>[2x]MTDTDTVEQFIHTIFARVTDDHGRPVDITAALPLLKQILTGYTQEVAEHKFNYIGESAVQFAMHLILADHFSKYENGCLSAIAKKYTVPLQLYKLIGKQIHLKEYVRPVYLKETLDMIVGILFRCYGITAVYKFIQEEFILLVNQDINNANSPKKPSSPSLSTNQADNPVKLLHELIQAKSGTLEAEAHETEDKKWEVKIVAKLNEKALPFSHARTNASKQKAKTEASRDILTYFTNYPDVCQHLQ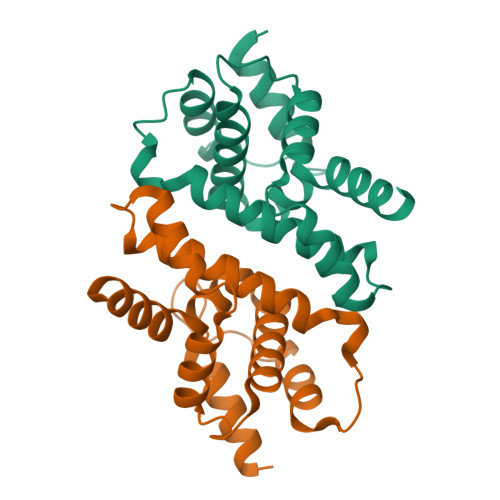VPVEGEVEIHVLPISENDYCHLFAET>EDKITVHFINRDGETLTTKGKIGDSLLDVVVQNNLDIDGFGACEGTLACSTCHLIFEQHIFEKL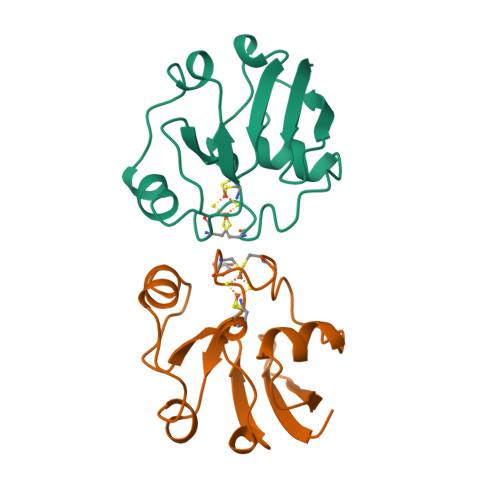EAITDEENDMLDLAYGLTDRSRLGCQICLTKAMDNMTVRVP[2x]> QPIFLNVLEAIEPGVVCAGHDNNQPDSFAALLSSLNELGERQLVHVVKWAKALPGFRNLHVDDQMAVIQYSWMGLMVFA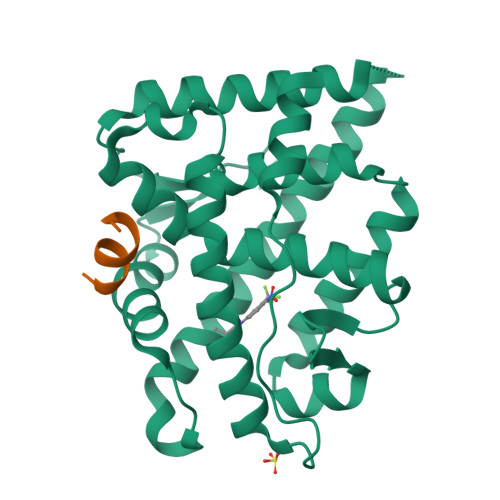MGWRSFTNVNSAMLYFAPDLVFNEYRMHKSRMYSQCVRMRHLSQEFGWLQITPQEFLCMKALLLFSIIPVDGLKNQKFFDELRMNYIKELDRIIACKRKNPTSCSRRFYQLTKLLDSVQPIARELHQFAFDLLIKSHMVSVDFPEMMAEIISVQVPKILSGKVKPIYFHTQ;> SDSAFSRLYTRS> PALISRLGALQQIIDDTPGIRLRTLSFDAARN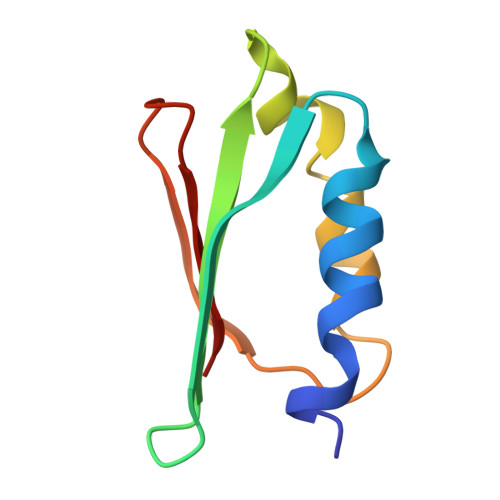ALQLEISAVSSQALEQFSQRARARFRVQTGEMKPRADGIEGRLTLEGA>GPGGSSMGTLGARRGLEWFLGFYFLSHIPITLLMDLQGVLPRDLYPVELRNLQQWYIEEFKDPLLQTPPAWFKSFLFCELVFQLPFFPIAAYAFFKGGCKWIRTPAIIYSVHTMTTLIPILSTLLLDDFSKASHFRGQGPKTFQERLFLISVYIPYFLIPLILLLFMVRNPYYK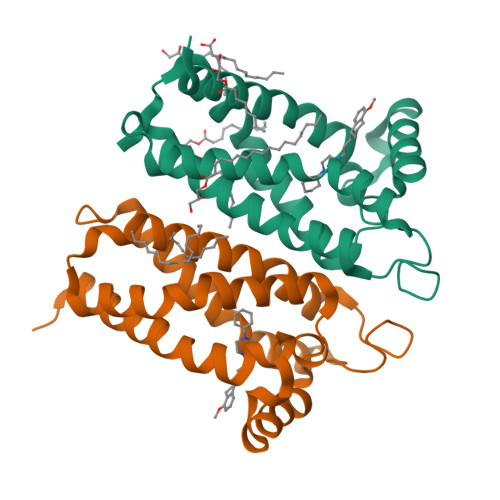[4x]> MSYVHPYGSTLPENGVIGRGYA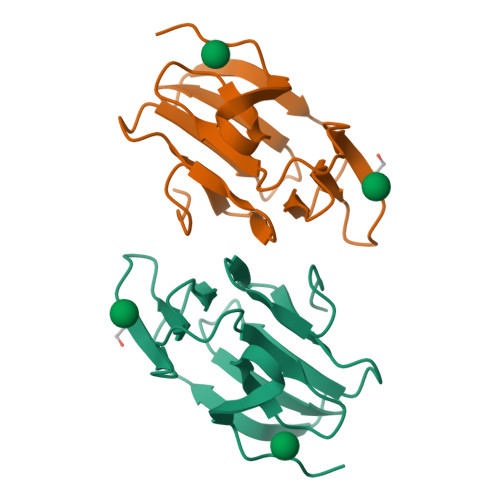LISDSGRVEFRVTDEGNIQLFLDDSRKLWSVDGKNASFVKMQTDGNCVGYDPNGTAVWHTATNGDDHPYNLVCQNDGNLVVYAKGGKAVWHTNTAVVH> GFPTELKPGTNQFLTTDDGVSAPILPNFHPTPCIHIPGEVRNLLELCQVETILEVNNVPTNATSLMERLRFPVSAQAGKGELCAVFRADPGRSG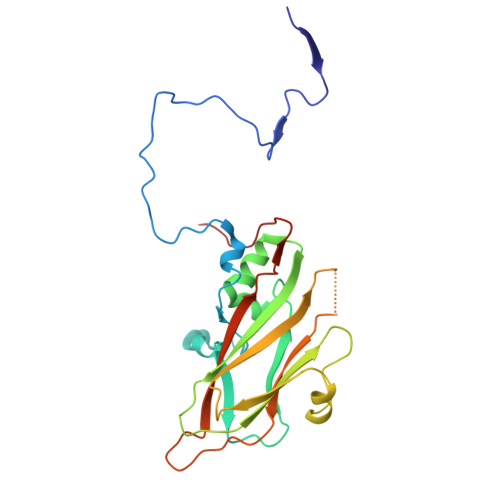PWQSTLLGQLCGYYTQWSGSLEVTFMFTGSFMATGKMLIAYTPPGGPLPKDRATAMLGTHVIWDFGLQSSVTLVIPWISNTHYRAHARDGVFDYYTTGLVSIWYQTNYVVPIGAPNTAYIIALAAAQKNFTMQLCKDASDILQTGTIQ>[2x]RGSHMETWVLGRRDVAEVVAAVGRDELMRRIIDRLTGGLAEIGRGERHLSPLRGGLERSEPVPGIWEWMPHREPGDHITLKTVGYSPANPARFGLPTILGTVARYDDTTGALTALMDGVLLTALRTGAASAVASRLLARPDSHTLGLIGTGAQAVTQLHALSLVLPLQRALVWDTDPAHRESFARRAAFTGVSVEIAEPARIAAEADVISTATSVAVGQGP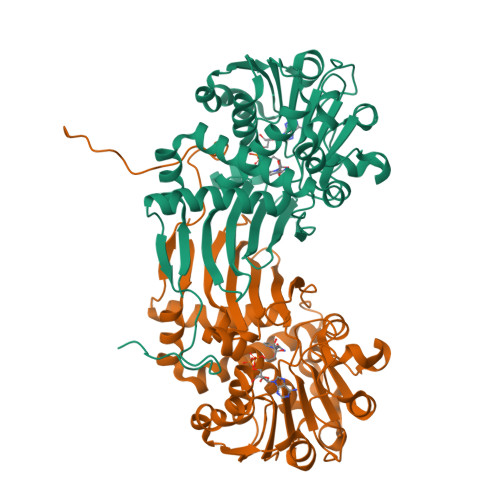VLPDTGVREHLHINAVGADLVGKTELPLGLLERAFVTADHPEQALREGECQQLSADRLGPQLAHLCADPAAAAGRQDTLSVFDSTGFAFEDALAMEVFLEAAAERDLGIRVGIEHHPGDALDPYALQPLPLPLAAPAH>MKKFIFATIFALASCAAQPAMAGYDKDLCEWSMTADQTEVETQIEADIMNIVKRDRPEMKAEVQKQL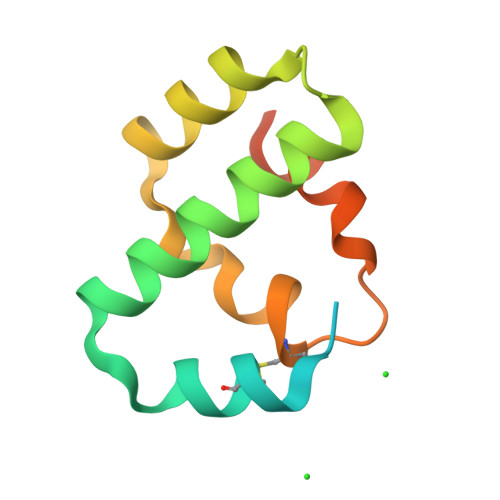KSGGVMQYNYVLYCDKNFNNKNIIAEVVGELEHHHHHH[2x]Found in both prokaryotes and eukaryotes, aldehyde dehydrogenases (ALDH) (EC 1.2.1.3) constitute a large family of NAD(P)-dependent enzymes with molecular weights of 50–60 kDa. ALDHTt contains an unusually extended C-terminal arm forming novel interactions with the N-terminus in the quaternary structure which interacts closely with the substrate entry tunnel. The ALDHTt monomer is composed of the three domains common to all ALDHs: (i) The NAD(P)+ binding domain (1–125 + 148–261) comprising a Rossman fold, (ii) the catalytic domain (267–458) and (iii) the oligomerization domain (126–147 + 494–501). However, the presence in ALDHTt of an unusual extended arm that wrap the facing monomer through H-bonds and salt bridges shows for the first time how the tetramer is not merely a dimer-of-dimers carrying out their functions independent of each other, but that the interaction of the N- and C-termini in CS-related monomers may regulate active site access in NCS-related molecules.

To probe the significance of the tail and its fulcrum points, two truncated tail mutants were made: (i) ALDHTt515 which removes all residues distal to the “Crook & Hook” and (ii) ALDHTt508, a mutant which removes the “Crook & Hook” entirely but retains the “Notch” to try and model other tail containing ALDHs. However, ALDHTt mutants could only be crystalized in a closed and compact conformation. The ALDHTt508 structure is “open” as the “Crook” of the tail has been removed, but there is still no movement in the anchor loop to an open position. It is worthy to note that the electron density maps were of a reduced quality in the C-terminal region of the truncated mutants compared to the native or the full length recombinant proteins, highlighting the role of the extended C-terminal tail in stabilizing the overall structure. The similarity in tail orientation and active site regulatory loops between ALDHTt and its deletion mutant structures even without intermolecular interactions between the end of the tail and N-terminal interactions hints that active site access is regulated by additional domain interactions. Interestingly, both truncated mutants ALDHTt508 and ALDHTt515 were slightly more active (specific activity of 1.068 ± 0.004 and 1.069 ± 0.012 U mg−1, respectively) than the recombinant wild type enzyme at 50 °C (0.965 ± 0.043 U mg−1), perhaps due to the presence of small amounts of ammonium sulfate acting as a stabilizing agent. Attempts to assess enzymatic activities at the higher temperature of 85 °C were not successful as both mutants rapidly lost their function compared to ALDHTt530 where it was still active up to 4 min, consistent with the Tm of ALDHTt530 of 84 °C. Taken together, the relative stability of the recombinant enzymes was in the order ALDHTt530 > ALDHTt515 ≈ ALDHTt508.

>MHHHHHHRKAAGKYGNTLEFGHLVGGEEVLEGPLLERRNPSDREDVVARFPEADKDLVRKAALKAREAFAEWSRTPAPIRGQVLFNLVKILEREKPTLTRLMVREVGKTPKEAAGDVQEAIDTALFFASEGRRLYGQTVPSEMRDKELFTFRRPLGVVGIITAGNFPIAVPSWKLIPAVLTGNTVVWKPSEDAPTLSFVFAKLFEEAGLPPGVLNVVFGGGKGSTGQWMVELMDEGLFQKFAFTGSTQVGRWIGEVAGRNLIRPTLELGGKNPLVVMRDADLDLAVEGAWWSAFATGGQRCTSAGNILVDAPIYEEFKRRFLERVEATLVGNPLLHPEVTYGPFINERFFARWQEHYRVGEAEGARLLFGRGRITRENPYPRFLGDPEAGLYGWPTVWEVRPGTRLFTEEVFGPTINLVKVDGIEEAIAVANSTPYGLSSAIYTNHRHWAYLFKVGIRAGMTSINNATVGAEAHLPFGGVKASGNGGRESGIWVLEEYTYWHAVNEEYSGRLQLAQM[2x]> MSRRRHSDENDGGQPHKRRKTSDANETEDHLESLICKVGEKSACSLESNLEGLAGVLEADLPNYKSKILRLLCTVARLLPEKLTIYTTLVGLLNARNYNFGGEFVEAMIRQLKESLKANNYNEAVYLVRFLSDLVNCHVIAAPSMVAMFENFVSVTQEEDVPQVRRDWYVYAFLSSLPWVGKELYEKKDAEMDRIFANTESYLKRRQKTHVPMLQVWTADKPHPQEEYLDCLWAQIQKLKKDRWQERHILRPYLAFDSILCEALQHNLPPFTPPPHTEDSVYPMPRVIFRMFDYTDDPEGPVMPGSHSVERFVIEENLHCIIKSHWKERKTCAAQLVSYPGKNKIPLNYHIVEVIFAELFQLPAPPHIDVMYTTLLIELCKLQPGSLPQVLAQATEMLYMRLDTMNTTCVDRFINWFSHHLSNFQFRWSWEDWSDCLSQDPESPKPKFVREVLEKCMRLSYHQRILDIVPPTFSALCPANPTCIYKYGDESSNSLPGHSVALCLAVAFKSKATNDEIFSILKDVPNPNQDDDDDEGFSFNPLKIEVFVQTLLHLAAKSFSHSFSALAKFHEVFKTLAESDEGKLHVLRVMFEVWRNHPQMIAVLVDKMIRTQIVDCAAVANWIFSSELSRDFTRLFVWEILHSTIRKMNKHVLKIQKELEEAKEKLARQHKRRSDDDDRSSDRKDGVLEEQIERLQEKVESAQSEQKNLFLVI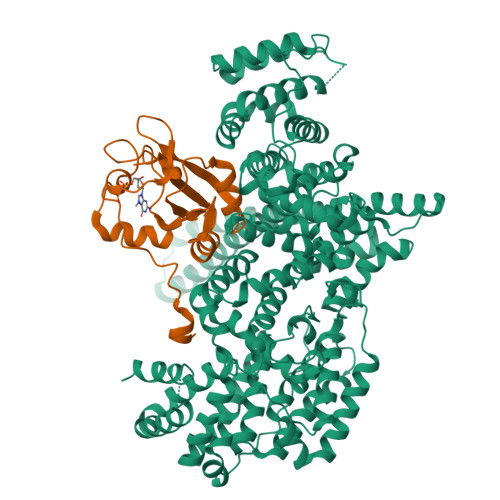FQRFIMILTEHLVRCETDGTSVLTPWYKNCIERLQQIFLQHHQIIQQYMVTLENLLFTAELDPHILAVFQQFCALQA;> MSGGLLKALRSDSYVELSQYRDQHFRGDNEEQEKLLKKSCTLYVGNLSFYTTEEQIYELFSKSGDIKKIIMGLDKMKKTACGFCFVEYYSRADAENAMRYINGTRLDDRIIRTDWDAGFKEGRQYGRGRSGGQVRDEYRQDYDAGRGGYGKLAQNQ> XFSPAA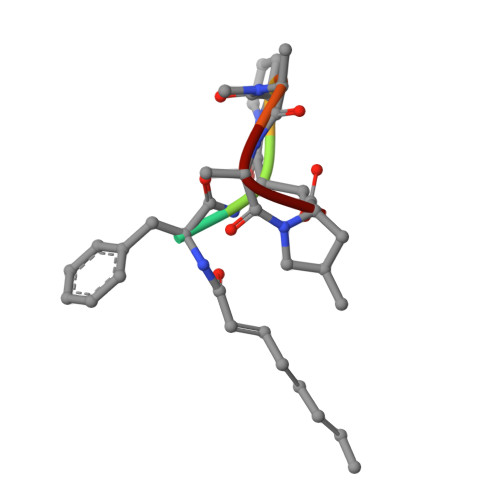P>GSHMGESPKFVRLRGLPWSATHKEILDFLENVNVTNGSAGIHLV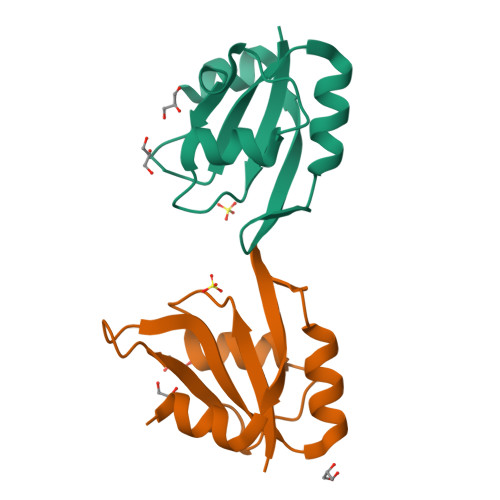TSRVDGKNTGEAYVEVASQEDVEEARKLNKASMGHRYIEVFTATPKEAKEAMRKISG[2x]>[2x]MFEQRVNSDVLTVSTVNSQDQVTQKPLRDSVKQALKNYFAQLNGQDVNDLYELVLAEVEQPLLDMVMQYTRGNQTRAALMMGINRGTLRKKLKKYGMN

Fis is one of a handful of nucleoid-associated proteins that bind prolifically throughout bacterial chromosomes. Fis regulates transcription, recombination, and replication reactions and is implicated in chromosome packaging. Multiple X-ray crystal structures of Fis-DNA complexes reveal that most of the Fis contacts are to the DNA backbone and extend over a 21 bp segment. The importance of the A/T-rich center (-2 to +2) is due to the requirement for a compressed minor groove, which enables the recognition helices in the Fis dimer to contact the consecutive major grooves.

We first tested the effects of individually substituting base pairs flanking the core at positions ±8, ±9, and ±10 in the context of the high affinity F1 site. These data indicate that the base at ±8 can have a large effect on Fis binding with a G being strongly inhibitory (150-fold poorer binding) and an A being moderately inhibitory (10-fold poorer binding). We determined X-ray structures of Fis complexes for each of the ±8 variants to elucidate the structural origins of the observed binding and lifetime differences. There are few differences in the overall structures of the proteins (RMSDs within 0.27 Å) and DNAs (RMSDs within 0.36 Å) in pairwise comparisons between the F1, F1±8C, F1±8A, and F1±8G complexes. In contrast, the phosphates at positions ±7 and ±6 are shifted by up to 0.6 Å in F1±8G and F1±8A, but by only 0.2 Å in the F1±8C complex. We suggest that a G/C or A/T bp at ±8 may increase the cost required to assume a DNA conformation that allows for the formation of the critical contacts to the ±8 phosphate. The magnitude of the shift in the DNA backbone between ±6 and ±8 correlates qualitatively with the effects of the ±8 substitutions on binding affinity, complex stability, and DNA bending. Another notable difference between the F1 and each of the ±8 variant structures is the van der Waals contact with the ±8 thymine methyl group made by the Arg85 guanidinium group and the Thr75 γ-hydroxyl group. These contacts are absent in the F1±8A, F1±8C, and F1±8G structures, but the positions of the Arg85 and Thr75 side chains are unchanged. DNA curvature of the Fis-bound complex is reduced by 12 and 17% for the ±8 purine substitutions (±8A and ±8G, respectively), whereas bending by the ±8C substitution is similar to F1. The DNA within the crystal structures of F1±8G as well as F1±8A reveal up to a 0.6 Å shift in the DNA backbone at the ±(6–7) and ±(7–8) phosphates, the latter of which is contacted by Fis-Arg89.5-METHYL-2'-DEOXYCYTIDINE 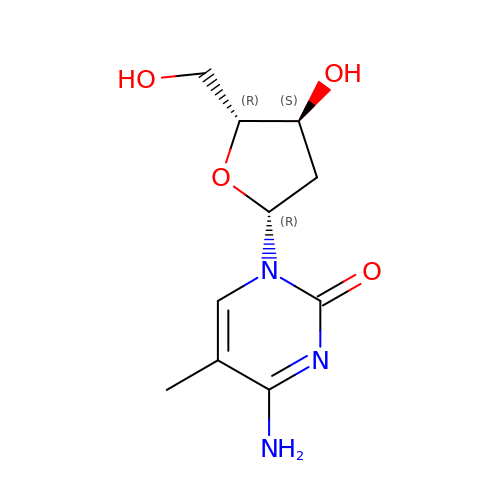| C10 H15 N3 O4 | LUCHPKXVUGJYGU-XLPZGREQSA-N>MTRHHHHHHGGGDYKDDDDKGGGKVPVEEEIQDLKAVWVELSNTWQEIDSLKETAWSAIIPRKVRKSLEDTLQKLKNLPNRIRQYSAFDHAQNLIKIYLKGNAIITDLHSEAIKDRHWKILKKRLNTNWIITELTLGSIWDSDLARNENIYREVITAAQGEIALEEFLKGVREFWTTLELDLVNYQRKCKLVRGWDDLFNKLAEHLNSISAMKMSPYYKVFEEEANHWDDRLNKVRSLLDVWIDVQRRWVYLEGIFSGSGDINQLLPAESTRFKSINSEFIAILKKVSGAPLILEVLAIERIQQTMERLSDLLGKVQKALGEYLERQRSAFARFYFVGDEDLLEIIGNSKDIIKIQKHFRKMFAGLANLTLDDEKTTIIGMSSAEGETVTFKKPISIANGPKIHEWLTMVESEMKSTLATLLSESLQHFNQVDVNDHSKYSEWVDNYPTQLVLLTSQIVWSTQVDQALGGGTLQQSKIQEQLQSIEQTTQMILNNLADSVLQDLSAQKRKKFEHLITELVHQRDVVRQLQKCKNLTGNKDFDWLYHMRYYYDATQENVLHKLVIHMANATFYYGFEYLGIGERLVQTPLTDRCYLTLTQALESRMGGNPFGPAGTGKTETVKALGSQLGRFVLVFCCDEGFDLQAMSRIFVGLCQCGAWGCFDEFNRLEERILSAVSQQIQTIQVALKENSKEVELLGGKNISLHQDMGIFVTMNPGYAGRSNLPDNLKKLFRSMAMIKPDREMIAQVMLYSQGFKTAEVLAGKIVPLFKLCQEQLSAQSHYDFGLRALKSVLVSAGGIKRKCQPPQLPPITDAESKTKADQIYCQYEIGVLLNSINDTMIPKLVADDIPLIQSLLLDVFPGSQLQPIQMDQLRKKIQEIAKQRHLVTKQEWVEKILQLHQILNINHGVMMVGPSGGGKTTSWEVYLEAIEQVDNIKSEAHVMDPKAITKDQLFGSLDLTTREWTDGLFTATLRRIIDNVRGESTKRHWIIFDGDVDPEWVENLNSLLDDNKLLTLPNGERLALPNNVRVMFEVQDLKYATLATISRCGMVWFSEEILTTQMIFQNYLDTLSNEPFDPQEKEQQKRNENAQLQQQQQTTITSPILTSPPTTSSSSRSTTSTTSMIPAGLKVQKECAAIISQYFEPGGLVHKVLEDAGQRPHIMDFTRLRVLNSFFSLMNRSIVNVIEYNQLHSDFPMSPENQSNYITNRLLYSLMWGLGGSMGLVERENFSKFIQTIAITPVPANTIPLLDYSVSIDDANWSLWKNKVPSVEVETHKVASPDVVIPTVDTTRHVDVLHAWLSEHRPLILCGPPGSGKTMTLTSTLRAFPDFEVVSLNFSSATTPELLLKTFDHHCEYKRTPSGETVLRPTQLGKWLVVFCDEINLPSTDKYGTQRVITFIRQMVEKGGFWRTSDHTWIKLDKIQFVGACNPPTDAGRVQLTHRFLRHAPILLVDFPSTSSLTQIYGTFNRALMKLLPNLRSFADNLTDAMVEFYSESQKRFTPDIQAHYIYSPRELSRWDRALLEAIQTMDGCTLEGLVRLWAHEALRLFQDRLVETEEKEWTDKKIDEVALKHFPSVNLDALKRPILYSNWLTKDYQPVNRSDLREYVKARLKVFYEEELDVPLVLFNEVLDHILRIDRVFRQPQGHALLIGVSGGGKSVLSRFVAWMNGLSIYTIKVNNNYKSSDFDDDLRMLLKRAGCKEEKICFIFDESNVLESSFLERMNTLLAGGEVPGLFEGEEFTALMHACKETAQRNGLILDSEEELYKYFTSQVRRNLHVVFTMNPASPDFHNRSATSPALFNRCVLDWFGEWSPEALFQVGSEFTRNLDLENPQYIAPPVFIQEAEIMGNNLMAIPPSHRDAVVSSLVYIHQTIGEANIRLLKRQGRQNYVTPRHYLDFINQVVLLINEKRDQLEEEQLHLNIGLKKLRDTEAQVKDLQVSLAQKNRELDVKNEQANQKLKQMVQDQQAAEIKQKDARELQVQLDVRNKEIAVQKVKAYADLEKAEPAIIEAQEAVSTIKKKHLDEIKSLPKPPTPVKLAMEAVCLMLGGKKLEWADIRKKIMEPNFITSIINYDTKKMMTPKIREAITKGYLEDPGFDYETVNRASKACGPLVKWATAQTYYSEILDRIKPLREEVEQLENAANELKLKQDEIVATITALEKSIATYKEEYATLIRETEQIKTESSKVKNKVDRSIALLDNLNSERGRWEQQSENFNTQMSTVVGDVVLASAFLAYIGFFDQNFRTDLMRKWMIRLDSVGIKFKSDLSVPSFLSKPEERLNWHANSLPSDELCIENAIMLKRFNRYPLVIDPSGQAMEFLMNQYADKKITKTSFLDSSFMKNLESALRFGCPLLVQDVENIDPVLNPVLNKEIRKKGGRILIRLGDQDVDFSPSFMIFLFTRDPTAHFTPDLCSRVTFVNFTVTPSSLQSQCLHEALKTERPDTHKKRSDLLKIQGEFQVKLRILEKSLLNALSQASGNILDDDSVISTLETLKKETTEIALKVEETETVMQEISEVSALYNPMALSCSRVYFAMEELSQFHLYQFSLRAFLDIFYNLLNNNPNLVDKKDPNERLVYLSKDIFSMTFNRVTRTLLNDDKLTFALQLTIISVKGTSNEIEESEWDFLLKGGDNLTSIKETIPQLDSLLSTTQQKWLICLRQQVPSFSKLVDHIQQNSSDWKQFFGKDQVGEPIIPESWIVAQAQLSNQQSTIVSNFRKILLMKAFHSDRVLQYSHSFVCSVFGEDFLNTQELDMANIVE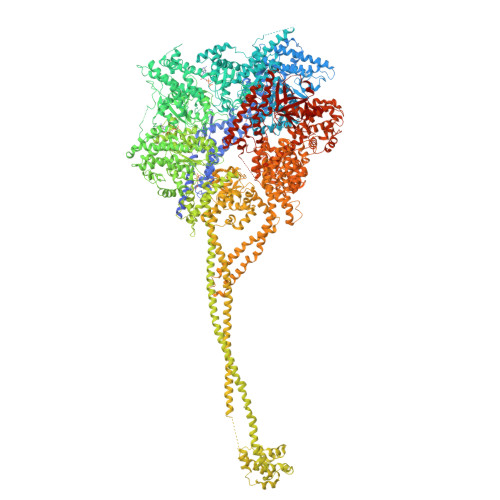KEVKSSSPLLLCSVPGYDASSKVDDLALQLHKQYKSFAIGSPEGFELAEKSIYAAAKSGTWVLLKNIHLAPQWLVQLEKKLHSLSPHPSFRLFMTSEIHPALPANLLRMSNVFSYENPPGVKANLLHTFIGIPATRMDKQPAERSRIYFLLAWFHAIIQERLRYIPLGWTKFFEFNDADLRGALDSIDYWVDLYSKGRSNIDPDKIPWIAVRTILGSTIYGGRIDNEFDMRLLYSFLEQLFTPSAFNPDFPLVPSIGLSVPEGTTRAHFMKWIEALPEISTPIWLGLPENAESLLLSNKARKMINDLQKMQSSEEDGEDDQVSGSSKKESSSSSSEDKGKAKLRATITEWTKLLPKPLKQLKRTTQNIKDPLFRCFEREISTGGKLVKKITNDLANLLELISGNIKSTNYLRSLTTSISKGIVPKEWKWYSVPETISLSVWISDFSKRMQQLSEISESSDYSSIQVWLGGLLNPEAYITATRQSASQLNGWSLENLRLHASSLGKISSEGGASFNVKGMALEGAVWNNDQLTPTDILSTPISIATLTWKDKDDPIFNNSSSKLSVPVYLNETRSELLFSIDLPYDQSTSKQNWYQRSVSISSWKSDI[2x]>MATSSMSKGCFVFKPNSKKRKISLPIEDYFNKGKNEPEDSKLRFETYQLIWQQMKSENERLQEELNKNLFDNLIEFLQKSHSGFQKNSRDLGGQIKLREIPTAALVLGVNVTDHDLTFGSLTEALQNNVTPYVVSLQAKDCPDMKHFLQKLISQLMDCCVDIKSKEEESVHVTQRKTHYSMDSLSSWYMTVTQKTDPKMLSKKRTTSSQWQSPPVVVILKDMESFATKVLQDFIIISSQHLHEFPLILIFGIATSPIIIHRLLPHAVSSLLCIELFQSLSCKEHLTTVLDKLLLTTQFPFKINEKVLQVLTNIFLYHDFSVQNFIKGLQLSLLEHFYSQPLSVLCCNLPEAKRRINFLSNNQCENIRRLPSFRRYVEKQASEKQVALLTNERYLKEETQLLLENLHVYHMNYFLVLRCLHKFTSSLPKYPLGRQIRELYCTCLEKNIWDSEEYASVLQLLRMLAKDELMTILEKCFKVFKSYCENHLGSTAKRIEEFLAQFQSLDAETKEEEDASGSQPKGLQKTDLYHLQKSLLEMKELRRSKKQTKFEVLRENVVNFIDCLVREYLLPPETQPLHEVVYFSAAHALREHLNAAPRIALHTALNNPYYYLKNEALKSEEGCIPNIAPDICIAYKLHLECSRLINLVDWSEAFATVVTAAEKMDANSATSEEMNEIIHARFIRAVSELELLGFIKPTKQKTDHVARLTWGGC[4x];>MKRDKTSDLVEEYFEAHSSSKVLTSDRTLQKLKRAKLDQQTLRNLLSKVSPSFSAELKQLNQQYEKLFHKWMLQLHLGFNIVLYGLGSKRDLLERFRTTMLQDSIHVVINGFFPGISVKSVLNSITEEVLDHMGTFRSILDQLDWIVNKFKEDSSLELFLLIHNLDSQMLRGEKSQQIIGQLSSLHNIYLIASIDHLNAPLMWDHAKQSLFNWLWYETTTYSPYTEETSYENSLLVKQSGSLPLSSLTHVLRSLTPNARGIFRLLIKYQLDNQDNPSYIGLSFQDFYQQCREAFLVNSDLTLRAQLTEFRDHKLIRTKKGTDGVEYLLIPVDNGTLTDFLEKEEEEA[4x]

The first step in genome replication, the binding of the Origin Recognition Complex (ORC) at origins of DNA replication, triggers a series of highly coordinated steps leading to the assembly of pre-replicative complexes (pre-RCs) in a process that involves CDC6 binding to ORC. ORC and CDC6 then function as an ATP-dependent assembler that first recruits a ring-shaped MCM2-7 hexamer with bound Cdt1 to DNA, and then loads a second MCM2-7 hexamer in a head-to-head orientation, whereby this double hexamer is topologically linked to double-stranded DNA (reviewed in [O'Donnell et al., 2013; Siddiqui et al., 2013; Bell and Labib, 2016]). Here, we report the structure of human ORC in a functionally active, ATP-hydrolysis ready state, providing insight into ATP-dependent protein loading as well as DNA and CDC6 binding. The structure of HsORC reveals a remarkable similarity between two very different ATPases: the replication initiator ORC-CDC6 ATPase and the replication fork DNA polymerase clamp loader.

The other lobe consists of N-terminally truncated ORC2 and full-length ORC3. In contrast, HsORC2/3 is composed of AAA+-like subunits, but with no predicted ATPase activity. Although our crystals of the HsORC2/3 complex diffracted only to 6.0 Å, with four complexes in the asymmetric unit, we were able to obtain phases by molecular replacement using the DmORC subunits. The resulting electron-density map was clear enough to show a significant movement of helices in ORC3 compared to the DmORC structure. In addition, the position of the WHD of ORC2 would result in significant clashes for two of the four ORC2 copies present in the crystal. This indicated to us that the structures were suitable for docking into the HsORC cryoEM reconstruction. Moreover, Orc2 and Orc3 were predicted to contain an AAA+ fold, but these subunits do not have the residues that are important for ATP hydrolysis and thus are predicted to be ‘AAA+ like’.>MSSKPKPIEIIGAPFSKGQPRGGVEKGPAALRKAGLVEKLKETEYNVRDHGDLAFVDVPNDSPFQIVKNPRSVGKANEQLAAVVAETQKNGTISVVLGGDHSMAIGSISGHARVHPDLCVIWVDAHTDINTPLTTSSGNLHGQPVAFLLKELKGKFPDVPGFSWVTPCISAKDIVYIGLRDVDPGEHYIIKTLGIKYFSMTEVDKLGIGKVMEETFSYLLGRKKRPIHLSFDVDGLDPVFTPATGTPVVGGLSYREGLYITEEIYKTGLLSGLDI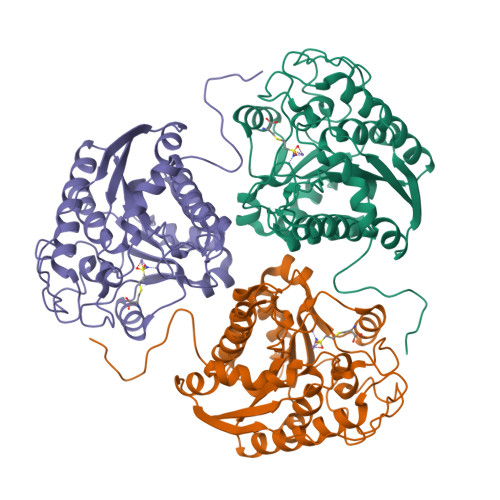MEVNPTLGKTPEEVTRTVNTAVALTLSCFGTKREGNHKPETDYLKPPK[3x]>[4x]AVNGKGMNPDYKAYLMAPLKKIPEVTNWETFENDLRWAKQNGFYAITVDFWWGDMEKNGDQQFDFSYAQRFAQSVKNAGMKMIPIISTHQCGGNVGDDCNVPIPSWVWNQKSDDSLYFKS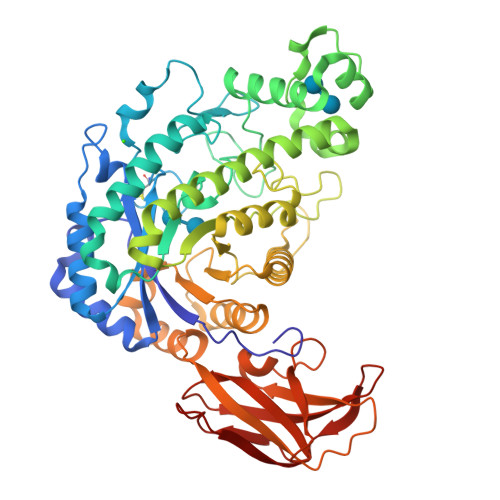ETGTVNKETLNPLASDVIRKEYGELYTAFAAAMKPYKDVIAKIYLSGGPAGELRYPSYTTSDGTGYPSRGKFQAYTEFAKSKFRLWVLNKYGSLNEVNKAWGTKLISELAILPPSDGEQFLMNGYLSMYGKDYLEWYQGILENHTKLIGELAHNAFDTTFQVPIGAKIAGVHWQYNNPTIPHGAEKPAGYNDYSHLLDAFKSAKLDVTFTCLEMTDKGSYPEYSMPKTLVQNIATLANEKGIVLNGENALSIGNEEEYKRVAEMAFNYNFAGFTLLRYQDVMYNNSLMGKFKDLLGVTPVMQTIVVKNVPTTIGDTVYITGNRAELGSWDTKQYPIQLYYDSHSNDWRGNVVLPAERNIEFKAFIKSKDGTVKSWQTIQQSWNPVPLKTTSHTSSW> MISNEEQTPLLKKINPTESTS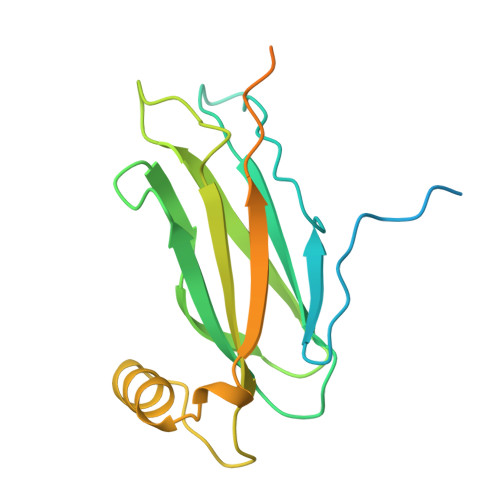KAEENEKVDSKVKAFKKPLSVFKGPLLHISPAEELYFGSTESGEKKTLIVLTNVTKNIVAFKVRTTAPEKYRVKPSNSSCDPGASVDIVVSPHGGLTVSAQDRFLIMAAEMEQSSGTGPAELTQFWKEVPRNKVMEHRLRCHTVESSKPNTLTLKDNAFNMSDKTSEDICLQLSRLLESNRKLEDQVQRHHHHHH>[2x]MADDQGCIEEQGVEDSANEDSVDAKPDRSSFVPSLFSKKKKNVTMRSIKTTRDRVPTYQYNMNFEKLGKCIIINNKNFDKVTGMGVRNGTDKDAEALFKCFRSLGFDVIVYNDCSCAKMQDLLKKASEEDHTNAACFACILLSHGEENVIYGKDGVTPIKDLTAHFRGDRCKTLLEKPKLFFIQACRGTELDDGIQAD;>SGPINDTDANPRYKIPVEADFLFAYS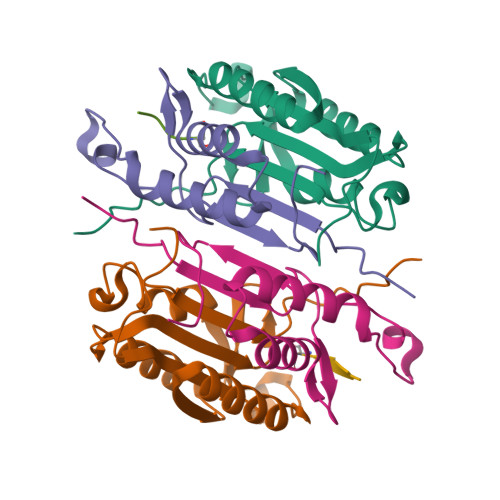TVPGYVSMRSPGRGSWFVQALCSILEEHGKDLEIMQILTRVNDRVARHFESCSDDPHFHEKKQIPCVVSMLTKELYFSQLEHHHHHH[2x];>[2x]XDEVD>[2x]MASMTGGQQMGRDPNSAFYKREM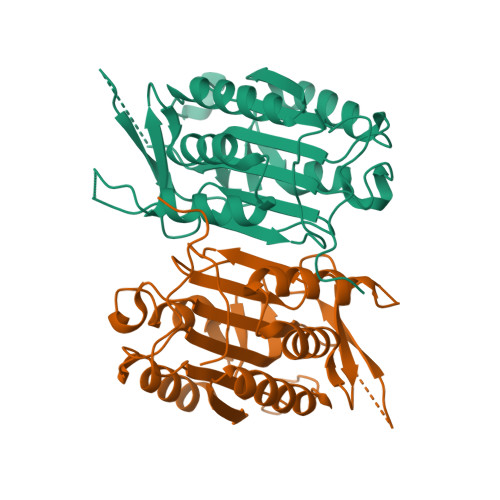FDPAEKYKMDHRRRGIALIFNHERFFWHLTLPERRGTCADRDNLTRRFSDLGFEVKCFNDLKVEELLLKIHEVSTVSHADADCFVCVFLSHGEGNHIYAYDAKIEIQTLTGLFKGDKCHSLVGKPKIFIIQAARGNQHDVPVIPLDVVDNQTEKLDTNITEVDAASVYTLPAGADFLMCYSVAEGYYSHRETVNGSWYIQDLCEMLGKYGSSLEFTELLTLVNRKVSQRRVDFCKDPSAIGKKQVPCFASMLTKKLHFFPKSNLEHHHHHH> ERRRGLTDPEMAAVILKALPEAPLDGNNKMGYFVTPRWKRLTEYEALTVYAQPNADWIAGGLDWGDWTQKFHGGRPSWGNETTELRTVDWFKHRDPLRRWHAPYVKDKAEEWRYTDRFLQGYSADGQIRAMNPTWRDEFINRYWGAFLFNEYGLFNAH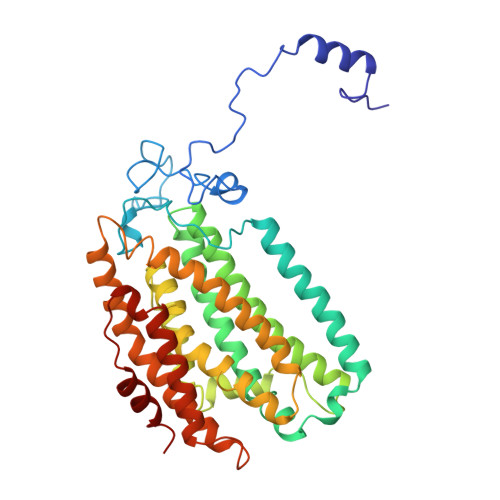SQGAREALSDVTRVSLAFWGFDKIDIAQMIQLERGFLAKIVPGFDESTAVPKAEWTNGEVYKSARLAVEGLWQEVFDWNESAFSVHAVYDALFGQFVRREFFQRLAPRFGDNLTPFFINQAQTYFQIAKQGVQDLYYNCLGDDPEFSDYNRTVMRNWTGKWLEPTIAALRDFMGLFAKLPAGTTDKEEITASLYRVVDDWIEDYASRIDFKADRDQIVKAVLAGLK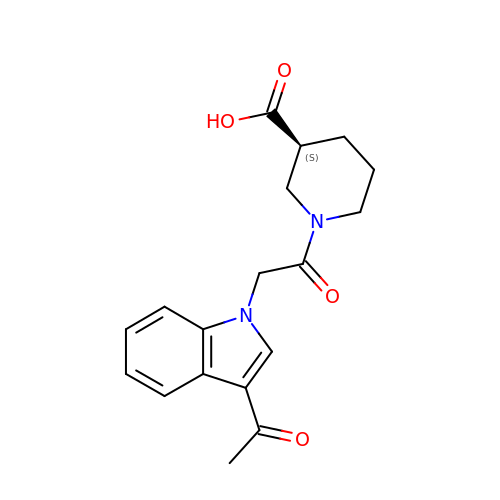(3S)-1-[2-(3-ethanoylindol-1-yl)ethanoyl]piperidine-3-carboxylic acid | C18 H20 N2 O4 | ZYTILVPFRSHVDL-ZDUSSCGKSA-N> MHHHHHHLV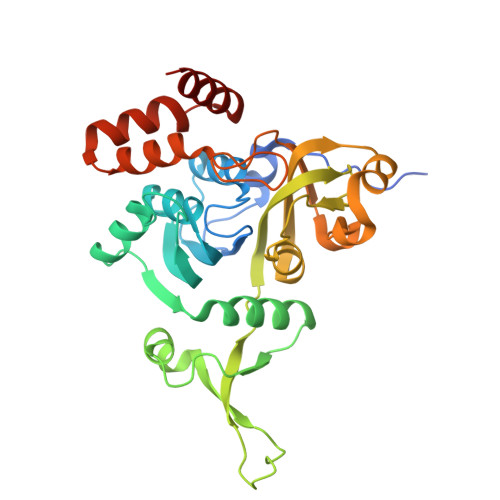PRGSVSKRDKRISLDDAVGELRSGMTIGIGGWGSRRKPMALVRALLRSDVTDLTVVTYGGPDLGLLCSAGKVTKAYYGFVSLDSAPFYDPWFAKARTAGEIAVREMDEGMVKCGLEAAAARLPFLPIRAGLGSDVRRFWGDELRTVTSPYPDASGKSETLIAMPALNLDAALVHLNLGDKHGNAAYTGVDPYFDDLYCAAAEKRFVSVERVVETEELVKTVPLQNLILNRMMVDGVVEAPNGAHFTLAGDSYGRDEKFQRHYAESAKTPQAWQQFVATYLSGSEDDYQAAVKKFAEEQA> MANVSKKVSWSGRDRDDEEAAPLLRRTARPGGGTPLLNGAGPGAARQSPRSALFRVGHMSSVELDDELLDPDMDPPHPFPKEIPHNEKLLSLKYESLDYDNSENQLFLEEERRINHTAFRTVEIKRWVICALIGILTGLVACFIDIVVENLAGLKYRVIKGNIDKFTEKGGLSFSLLLWATLNAAFVLVGSVIVAFIEPVAAGSGIPQIKCFLNGVKIPHVVRLKTLVIKVSGVILSVVGGLAVGKEGPMIHSGSVIAAGISQGRSTSLKRDFKIFEYFRRDTEKRDFVSAGAAAGVSAAFGAPVGGVLFSLEEGASFWNQFLTWRIFFASMISTFTLNFVLSIYHGNMWDLSSPGLINFG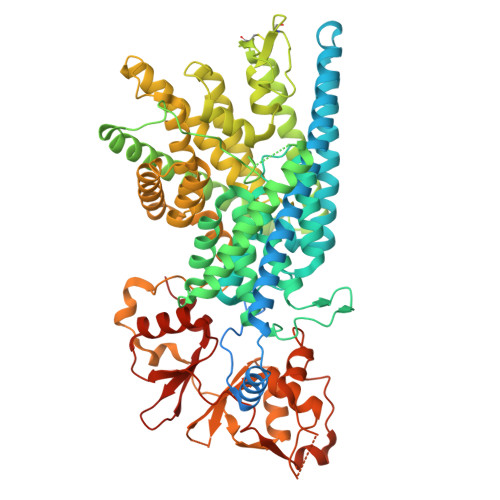RFDSEKMAYTIHEIPVFIAMGVVGGVLGAVFNALNYWLTMFRIRYIHRPCLQVIEAVLVAAVTATVAFVLIYSSRDCQPLQGGSMSYPLQLFCADGEYNSMAAAFFNTPEKSVVSLFHDPPGSYNPLTLGLFTLVYFFLACWTYGLTVSAGVFIPSLLIGAAWGRLFGISLSYLTGAAIWADPGKYALMGAAAQLGGIVRMTLSLTVIMMEATSNVTYGFPIMLVLMTAKIVGDVFIEGLYDMHIQLQSVPFLHWEAPVTSHSLTAREVMSTPVTCLRRREKVGVIVDVLSDTASNHNGFPVVEHADDTQPARLQGLILRSQLIVLLKHKVFVERSNLGLVQRRLRLKDFRDAYPRFPPIQSIHVSQDERECTMDLSEFMNPSPYTVPQEASLPRVFKLFRALGLRHLVVVDNRNQVVGLVTRKDLARYRLGKRGLEELSLAQT> XSAWSHPQFE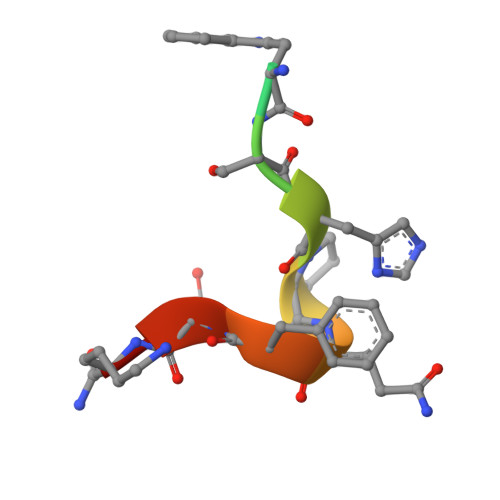KX>[2x]MNTNNIKKYAPQARNQFRDAVIQKLTTLGISADKKGNLQIADAELVGETMRYGQFDYPKSTLTRRDRLVKRAREQGFDVLVEHCAYTWFNRLCAIRYMEIHGYLDHGFHMLSHPDNPTGFEVLDHVPEVAEALLPEKKAQLVEMKLSGNQDEAIYRELLLAQCHALHRAMPFLFEAVDDEAELLLPDNLTRTDSILRGLVDGIPEEDWQEVEVIGWLYQFYISEKKDAVIGKVVKSEDIPAATQLFTPNWIVQYLVQNSVGRQWLQTYPDSPLKGKMDYYIEPAEQTPEVQAQLAAITPASIEPESIKVLDPACGSGHILIEVYNVLKNIYEERGYRARDIPQLILENNIFGLDIDDRAAQLSGFALLMMARQDDRRIFTRDVRLNIVSLQESLHLDIAKLWQQLNFHQQNQTGSMGDMFAENTALAHTDSAEYQLLMRTLKRFVNAKTLGSLIQVPQEEEAELKAFLEALYRMEQEGDFQQKAAAKAFIPYIQQAWILAQRYDAVVANPPYMGGKGMNSELKEFAKNNFPDSKADLFAMFMQNAFSLLKENGFNAQVNMQSWM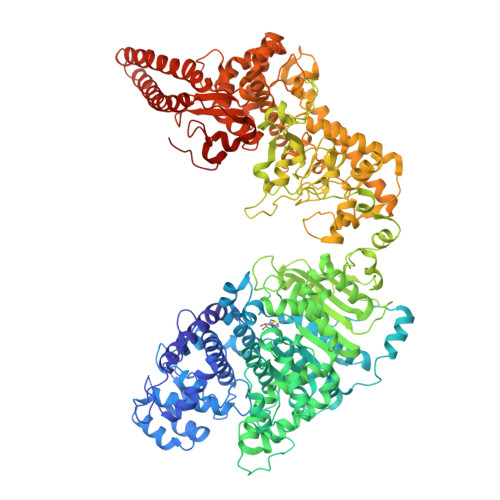FLSSYEALRNWLLDNKTFITMAHLGARAFGQISGEVVQTTAWVIKNQHSERYQPVFFRLIDGREEVKKSDLLLRKNIFDKFTQHDFKNIPGMPIAYWIDLPSLLSFRHHKKLGEKIALKAGMSTGDNIKFQRYWYEVSIKKTLITNKESNTKIDIHNIKWFPCSSGGEYRKWYGNNEIVVNWENNGYEIRNFKFENGKTRSAVRNDEYYFREGITWSKISQGNFCVRYRPKGFVFDDTGRCGFSNNKNELLYAAGLMCTPVVNHYLSILAPTLSFTSGELASVPYPEIEDEIIELVTNAIEIAKNDWDSQEQSWDYVCSPLLEHNSTQLLRNIYKQKINTNIKLVETLLLIENTINNIFIDKLQLDKTIIKAVLQSEITLLCNPNYRYKNIQDHTDLTNKYYTDITIDILSYIIGCMMGRYSLDREGLVYAHEGNKGFAELVAEDAYKTFPADNDGILPLMDDEWFDDDVTSRVKEFVRTVWGEEHLQENLEFIAESLCLYAIKPKKGESALDTIRRYLSTQFWKDHMKMYKKRPIYWLFSSGKEKAFECLVYLHRYNDATLARMRTEYVVPLLARYQANIDRLNEQVDGASGGEATRLKRERDSLSKKFNELRSFDDRLRHYADMRISIDLDDGVKVNYGKFGDLLADVKAITGNAPEII>HHHHHHMASSAQDGNNPLFSPYKMGKFNLSHRVVLAPMTRCRALNNIPQAALGEYYEQRATAGGFLITEGTMISPTSAGYPHVPGIFTKEQVREWKKIVDVVHAKGAVIFCQLWHVGRASHEVYQPAGAAPISSTEKPISNRWRILMPDGTHGIYPKPRAIGTYEISQVVEDYRRSALNAIEAGFDGIEIHGAHGYLIDQFLKDGINDRTDEYGGSLANRCKFITQVVQAVVSAIGADRVGVRVSPAIDYLDAMDSNPLSLGLAVVERLNKIQLHSGSKLAYLHVTQPRYVAYGQTEAGRLGSEEEEARLMRTLRNAYQGTFICSGGYTRELGIEAVAQGDADLVSYGRLFISNPDLVMRIKLNAP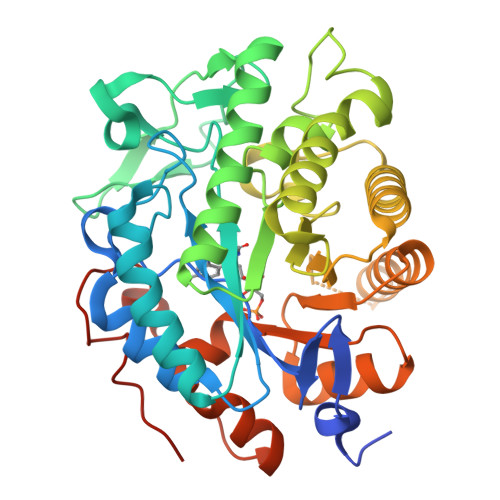LNKYNRKTFYTQDPVVGYTDYPFLQGNGSNGPLSRL[2x]> MRITFNDVKTSLGITESYDIVNAIRNSQGDNFKSYVPLATANNVAEVGAGILINQTVQNDFITSLVDRIGLVVIRQVSLNNPLKKFKKGQIPLGRTIEEIYTDITKEKQYDAEEAEQKVFEREMPNVKTLFHERNRQGFYHQTIQDDSLKTAFVSWG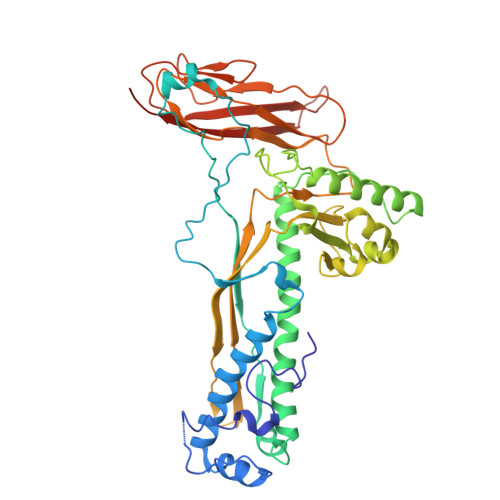NFESFVSSIINAIYNSAEVDEYEYMKLLVDNYYSKGLFTTVKIDEPTSSTGALTEFVKKMRATARKLTLPQGSRDWNSMAVRTRSYMEDLHLIIDADLEAELDVDVLAKAFNMNRTDFLGNVTVIDGFASTGLEAVLVDKDWFMVYDNLHKMETVRNPRGLYWNYYYHVWQTLSVSRFANAVAFVSGDVPAVTQVIVSPNIAAVKQGGQQQFTAYVRATNAKDHKVVWSVEGGSTGTAITGDGLLSVSGNEDNQLTVKATVDIGTEDKPKLVVGEAVVSIRPNNASGGAQA> MSLTNHTETITVEEGQTLT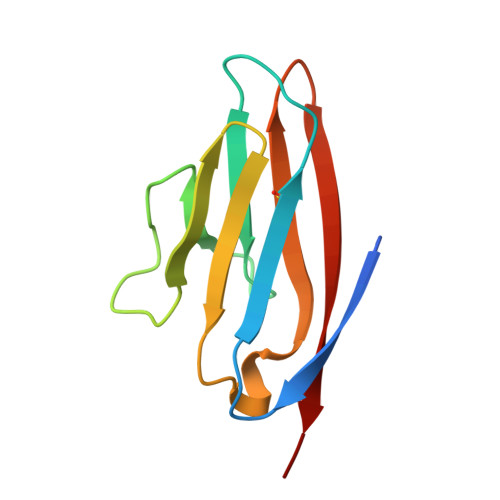LKCVTSLRKNSSLQWLTPSGFTIFLNEYPALKNSKYQLLHHSANQLSITVPNVTLQDEGVYKCLHYSDSVSTKEVKVIVLAT> GSHMEEPEETKQVSWKLVTQYALDTKCEDVFLLMGMYLNFQEAPAACAACAAADQPNHFNHHEKHYYNAQIFADSKNQKSICQQAVDTVAAKQRVDSLHMTREEMLVERFNFLLDKMDLIFGAHGNAVLEQYMAGVAWIHCLLPQMDTVIYEFLKCIVLNIPKKRYWLFKGPIDSGKTTLAAALLDLCGGKSLNVNMPLERLNFELGVGIDQFMVVFEDVKGTGAESRDLPSGHGISNLDCLRDYLDGSVKVNLERKHQNKRTQVFPPGIVTMNEYSVPRTLQARFVRQIDFRPKAYLRKSLSCSEYLLEKRILQS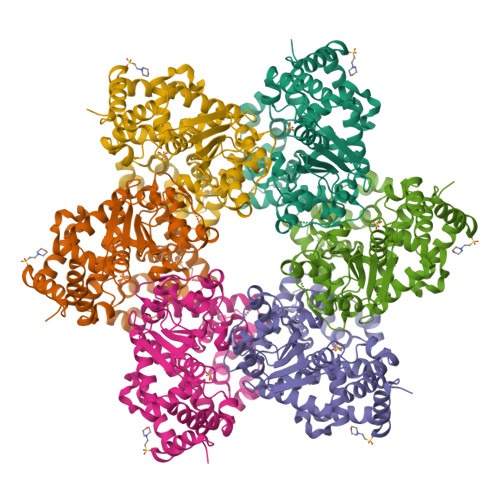GMTLLLLLIWFRPVADFAAAIHERIVQWKERLDLEISMYTFSTMKANVGMGAPILD> MPKLPRGLRFGADNEILNDFQELWFPDLFIESSDTHPWYTLKGRVLNAHLDDRLPNVGGRQVRRTPHRVTVPIASSGLRPVTTVQYDPAALSFLLNARVDWDFGNGDSANLVINDFLFRTFAPKEFDFSNSLVPRYTQAFSAFNAKYGTMIGEGLETIKYLGLLLRRLREGYRAVKRGDLRALRRVIQSYHNGKWKPATAGNLWLEFRYGLMPLFYDIRDVMLDWQNRHDKIQRLLRFSVGHGEDYVVEFDNLYPAVAYFKLKGEITLERRHRHGISYANREGYAVFDNGSLRPVSDWKELATAFINPHEVAWELTPYSFV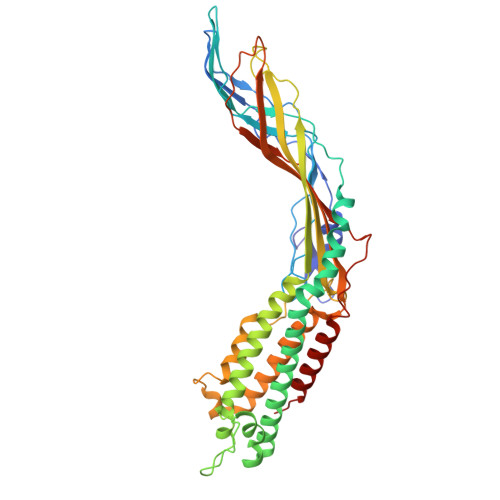VDWFLNVGDILAQQGQLYHNIDIVDGFDRRDIRLKSFTIKGERNGRPVNVSASLSAVDLFYSRLHTSNLPFATLDLDTTFSSFKHVLDSIFLLTQRVKR>GGGGGGGG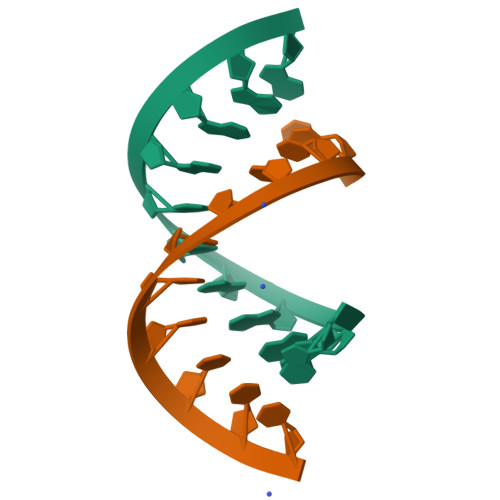GGG[2x];>CCCCCCCCCCC[2x]> 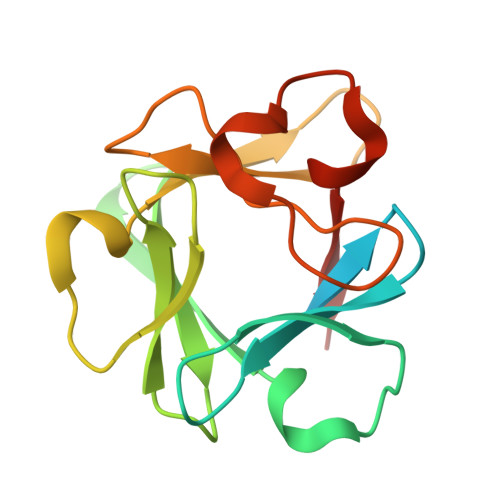AAGSITTLPALPEDGGSGAFPPGHFKDPKRLYCKNGGFFLRIHPDGRVDGVREKSDPHIKLQLQAEERGVVSIKGVSANRYLAMKEDGRLLASKSVTDECFFFERLESNNYNTYRSRKYTSWYVALKRTGQYKLGSKTGPGQKAILFLPMSAKS>MNNLKLDIVEQDDKAIVRVQGDIDAYNSSELKEQLRNFISTTSKKKI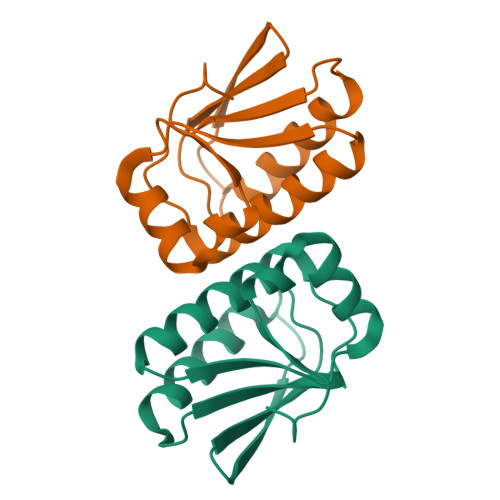VLDLSSVSYMDSAGLGTLVVILKDAKINGKEFILSSLKESISRILKLTHLDKIFKITDTVEEA[2x]> C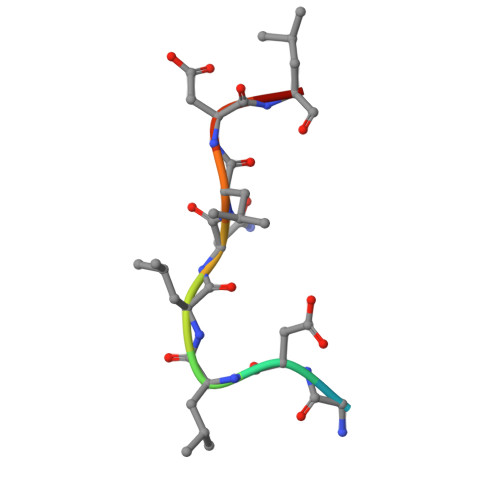GDLLNLDLG> EGGIDSGMMLQLEKN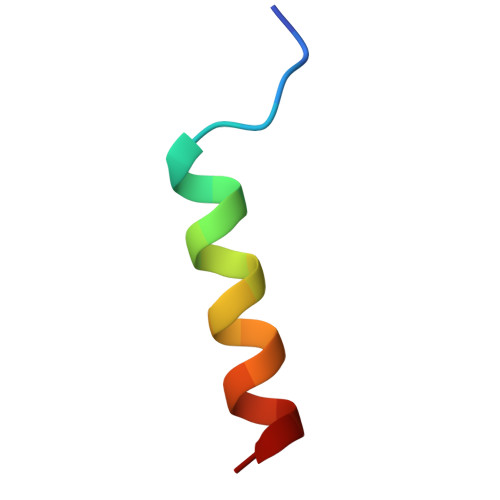LVDIVD>GPHMPEQYRYTLPVKAGEQRLLGELTGAACATLVAEIAERHAGPVVLIAPDMQNALRLHDEISQFTDQMVMNLADWETLPYDSFSPHQDIISSRLSTLYQLPTMQRGVLIVPVNTLMQRVCPHSFLHGHALVMKKGQRLSRDALRTQLDSAGYRHVDQVMEHGEYATRGALLDLFPMGSELPYRLDFFDDEIDSLRVFDVDSQRTLEEVEAINLLPAHEFPTDKAAIELFRSQWRDTFEVKRDPEHIYQQVSKGTLPAGIEYWQPLFFSEPLPPLFSYFPANTLLVNTGDLETSAERFQADTLARFENRGVDPMR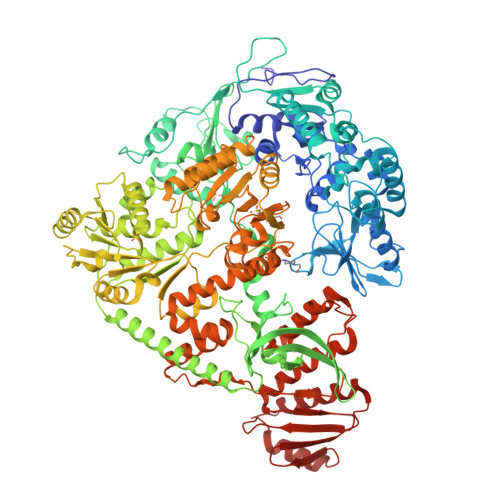PLLPPQSLWLRVDELFSELKNWPRVQLKTEHLPTKAANANLGFQKLPDLAVQAQQKAPLDALRKFLETFDGPVVFSVESEGRREALGELLARIKIAPQRIMRLDEASDRGRYLMIGAAEHGFVDTVRNLALICESDLLGERVARRRQDSRRTINPDTLIRNLAELHIGQPVVHLEHGVGRYAGMTTLEAGGITGEYLMLTYANDAKLYVPVSSLHLISRYAGGAEENAPLHKLGGDAWSRARQKAAEKVRDVAAELLDIYAQRAAKEGFAFKHDREQYQLFCDSFPFETTPDQAQAINAVLSDMCQPLAMDRLVCGDVGFGKTEVAMRAAFLAVDNHKQVAVLVPTTLLAQQHYDNFRDRFANWPVRIEMISRFRSAKEQTQILAEVAEGKIDILIGTHKLLQSDVKFKDLGLLIVDEEHRFGVRHKERIKAMRANVDILTLTATPIPRTLNMAMSGMRDLSIIATPPARRLAVKTFVREYDSMVVREAILREILRGGQVYYLYNDVENIQKAAERLAELVPEARIAIGHGQMRERELERVMNDFHHQRFNVLVCTTIIETGIDIPTANTIIIERADHFGLAQLHQLRGRVGRSHHQAYAWLLTPHPKAMTTDAQKRLEAIASLEDLGAGFALATHDLEIRGAGELLGEEQSGSMETIGFSLYMELLENAVDALKAGREPSLEDLTSQQTEVELRMPSLLPDDFIPDVNTRLSFYKRIASAKTENELEEIKVELIDRFGLLPDPARTLLDIARLRQQAQKLGIRKLEGNEKGGVIEFAEKNHVNPAWLIGLLQKQPQHYRLDGPTRLKFIQDLSERKTRIEWVRQFMRELEENAIA[2x]The largest of these factors, eIF3, is a multi-subunit complex consisting of five stoichiometric subunits in yeast (eIF3a, b, c, g and i). One of its large subunits, eIF3b, serves as a scaffold within eIF3 as it interacts with several other subunits. Here, by using X-ray crystallography we studied the structure of yeast eIF3b-RRM and showed that it corresponds to the canonical RNA recognition motif. The structure is composed of four β-strands and two α-helices which are arranged in a β-α-β-β-α-β sequential order.

Two different truncations of the N-terminal domain of yeast eIF3b were designed based on homology to the published structure of its human ortholog. The second construct encompassing residues 76–170 was designed to have an extra helix according to the secondary structure predictions. Highly reproducible crystals were obtained in space group P212121 with two molecules per asymmetric unit which diffracted to 1.25 Å. Crystallographic phases were obtained by molecular replacement using the structure of the sex-lethal RRM domain as search model. The last β-strand is followed by a short α-helix which connects this domain to the rest of the protein. The two yeast eIF3b76–170 monomers occupying the asymmetric unit are related by a two-fold non-crystallographic symmetry axis, forming a closely packed dimer. Two monomers in the asymmetric unit are held in place by interactions between their β-sheets and between each β-sheet and the extended α-helix of the neighboring chain. Interestingly, comparison of the dimer of eIF3b-RRM with hnRNP A1 (UP1) shows that Tyr 158, Asp 162 and Phe166 of one monomer interact with the RNP1 motif of the second monomer in the crystal, mimicking the presence of the oligonucleotide. Comparison of the relative orientation of the monomers between eIF3b-RRM76–170 and eIF3b-RRM76–161 showed that chain B in eIF3b-RRM76–161 has been displaced by ∼9 Å relative to the same chain in eIF3b-RRM76–170. Therefore this dimer is most probably an artifact of the crystallization and not the functional unit of the protein in the solution.

>[2x]GPLGSDQYIVVNGAPVIPSAKVPVLKKALTSLFSKAGKVVNMEFPIDEATGKTKGFLFVECGSMNDAKKIIKSFHGKRLDLKHRLFLYTMKDVERYNSDD> MNSDYILQHADALVKRVSKLIVNEPAARAALRRGVGLAPEDPRMLAAHRVVAPYVPVPTDYDVDRRRAASLWDVHAVERAFYAVAAIMAAQPRSARDQEAEATEEQTGEPQ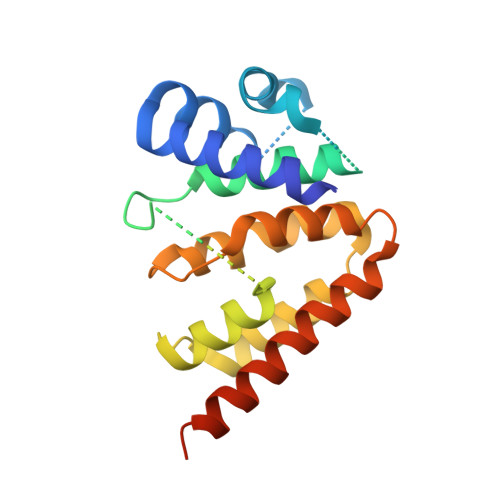DSEALTEPTPAEESSATKDGKPDRRPNLGVSLAQAVFDKGLNADSTEQRLHLIARQNLDGVHRHLPRLVLYLRSDQVHIDWGILIRDLARWGHTPRHVAREWVQDYHRTLETLTRQAEQKNKNNTTDEEAEAA> VFPSSVFVPDEWEVSREKITLLRELGQGSFGMVYEGNARDIIKGEAETRVAVKTVNESASLRERIEFLNEASVMKGFTCHHVVRLLGVVSKGQPTLVVMELMAHGDLKSYLRSLRPEAENNPGRPPPTLQE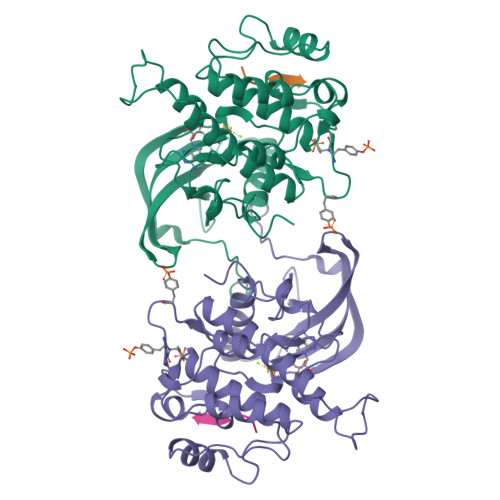MIQMAAEIADGMAYLNAKKFVHRDLAARNCMVAHDFTVKIGDFGMTRDIYETDYYRKGGKGLLPVRWMAPESLKDGVFTTSSDMWSFGVVLWEITSLAEQPYQGLSNEQVLKFVMDGGYLDQPDNCPERVTDLMRMCWQFNPKMRPTFLEIVNLLKDDLHPSFPEVSFFHSEENK;> KKKLPATGDYMNMSPVGD> MKPDETPMFDPSLLKE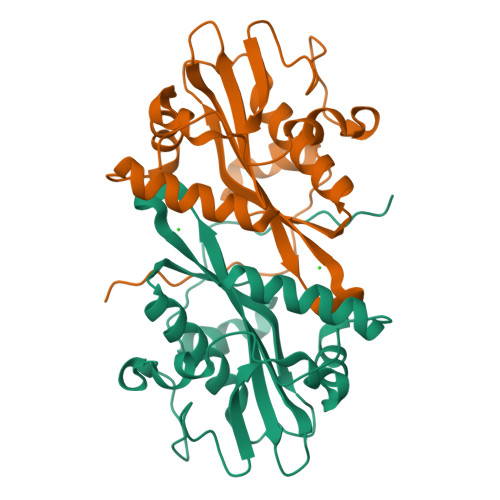VDWSQNTATFSPAISPTHPGEGLVLRPLCTADLNRGFFKVLGQLTETGVVSPEQFMKSFEHMKKSGDYYVTVVEDVTLGQIVATATLIIEHKFIHSCAKRGRVEDVVVSDECRGKQLGKLLLSTLTLLSKKLNCYKITLACLPQNVGFYKKFGYTVSEENYMCRRFLK> LAAGTPALGDDRGRPWPASLAALALDGKLRTDSNATAAASTDFGNITSALPAAVLYPSSTADLVALLSAANSTPGWPYTIAFRGRGHSLMGQAFAPGGVVVNMASLGDAAAPPRINVSADGRYVDAGGEQVWIDVLRASLARGVAPRSW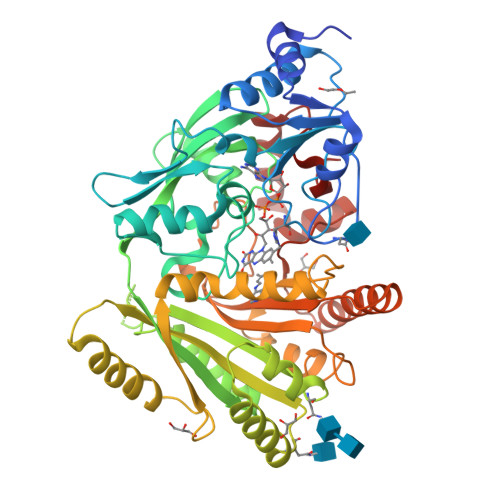TDYLYLTVGGTLSNAGISGQAFRHGPQISNVLEMDVITGHGEMVTCSKQLNADLFDAVLGGLGQFGVITRARIAVEPAPARARWVRLVYTDFAAFSADQERLTAPRPGGGGASFGPMSYVEGSVFVNQSLATDLANTGFFTDADVARIVALAGERNATTVYSIEATLNYDNATAAAAAVDQELASVLGTLSYVEGFAFQRDVAYAAFLDRVHGEEVALNKLGLWRVPHPWLNMFVPRSRIADFDRGVFKGILQGTDIVGQLIVYPLNKSMWDDGMSAATPSEDVFYAVSLLFSSVAPNDLARLQEQNRRILRFCDLAGIQYKTYLARHTDRSDWVRHFGAAKWNRFVEMKNKYDPKRLLSPGQDIFN> MTTRIALDPFVSDLEAESAALRAAGPLAAVELPGGVPVWAVTHHAEAKKLLTDPRLVKDINVWGAWQRGEIAPDWPLIGLANPGRSMLTV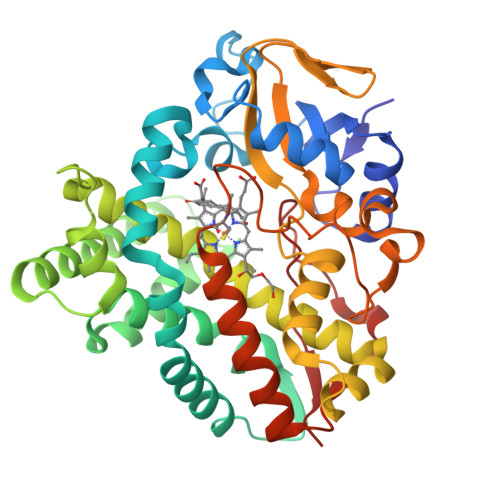DGADHRRMRTLVAQALTPRRVEQMRERITKLTEELLDRLTGEVVDLKADFAYPLPMYVVADLMGIDEARLPRLGELFEKFFSTQTPPAEVIATLTELAGIMAETVAAKRAAPGDDLTSALILASEDGDHLTDAEIVSTLQLMVAAGHETTISLIVNAVVNLSTHPEQRALVLSGEADWSSVVEETLRYSTPTSHVLIRFATEDVPVGDKVLPAGDALIVSYGALGRDEAAHGPTAGEFDITRSTENRHISFGHGPHVCPGAALSRLEAGVALPALYARFPKLDLAVPAAELRNKPVVTQNDLFELPVRLG> A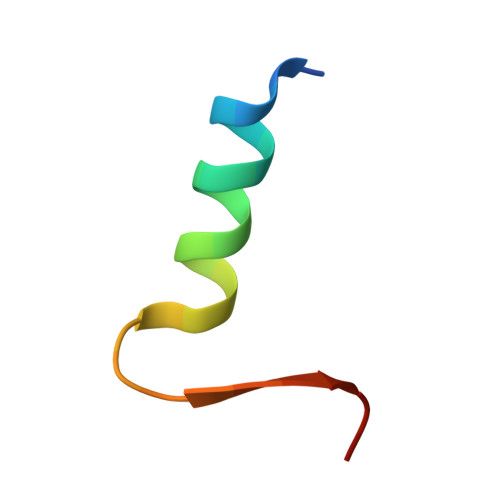STERKWAELARRIRGAGGVTLNGFG>[2x]TATGDEWWAKCKQVDVLDSEMSYYDSDPGKHKNTVIF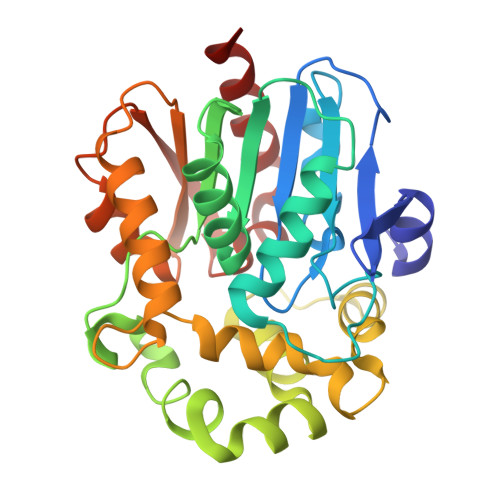LHGNPTSSYLWRNVIPHVEPLARCLAPDLIGMGKSGKLPNHSYRFVDHYRYLSAWFDSVNLPEKVTIVCHDWGSGLGFHWCNEHRDRVKGIVHMESVVSPLKGWESFPETARDILPQALRSEAGEEMVLKKNFFIERLLPSSIMRKLSEEEMDAYREPFVEPGESRRPTLTWPREIPIKGDGPEDVIEIVKSYNKWLSTSKDIPKLFINADPGFFSNAIKKVTKNWPNQKTVTVKGLHFLQEDSPEEIGEAIADFLNELTK> AAQLSEQLAELEKRSGGRLGVAVLDTATGRRIAYRGDERFPMCSTFKALLAAAVLARVDQGKERLDRRITYGKEDLVDYSPVTEKHVGDGMTVAELCEAAITLSDNTAANLLLEALGGPAALTAFLRSIGDEVTRLDRWEPELNEAAPGDPRDTTTPAAMAATLRTLLLGDALSPASRQQLVDWLVANKTGDKRLRAGLPADDRVGDKTGTGGHGTTNDIAVIWPPGRAPIVVTVYLTESQVDADARDAVIAEVGRLVVEAFHHHHHH

Here, we explore and test these notions using resurrected Precambrian β-lactamases11 as scaffolds for the engineering of completely new active sites. Of these systems, resurrected Precambrian β-lactamases have been thoroughly characterized in terms of their structure, function and stability. These putative ancestral proteins have been shown to be highly stable and able to efficiently degrade several antibiotics. A hydrophobic-to-ionizable amino acid replacement generates a buried (or partially buried) residue with the perturbed properties that are useful in catalysis and conformational flexibility assists the generation of a completely new active site by facilitating substrate and transition-state binding. We have shown that, when using resurrected Precambrian β-lactamases as scaffolds for protein engineering, a minimalist design approach based on this mechanism leads to levels of catalysis for the Kemp elimination reaction of up to approximately seven orders of magnitude above the rate of the uncatalysed reaction, as well as to significant ester hydrolysis activity.

Specifically, X-ray crystallography in the presence of 5(6)-nitrobenzotriazole, a known transition-state analogue of the Kemp elimination reaction and inhibition by this analogue support that Kemp elimination does occur at the site generated by the W229D replacement. Following from this, 3D-structure determination in the presence of the transition-state analogue confirms the role of conformational flexibility in the generation of a new function, as transition-state binding is shown to rely on conformational rearrangements. Specifically, the bound transition-state analogue is displaced with respect to the position originally occupied by the tryptophan 229, as required by the presence of an aspartate residue at position 229 in the active variants. Such a displacement is made possible by a shift of the h11 α-helix (and the concomitant shift of the substantially solvent-exposed h1 α-helix). We note also that the catalytic efficiency for the Kemp elimination in the engineered ancestral proteins correlates with the transition-state analogue binding constants derived from inhibition experiments, supporting that catalysis is linked to transition-state stabilization. We subsequently performed MD simulations in the presence of the transition-state analogue 5(6)-nitrobenzotriazole (TSA) to explore the impact of transition-state binding on the conformational dynamics, as well as how well each system could accommodate the transition state in its new active site. The W229D variants of the ancestral scaffolds that give rise to substantial Kemp elimination activity (PNCA, GNCAMP and GNCA4) can accept the TSA in the MD simulations, although the TSA dissociates from the less active W229D variant of the PNCA scaffold after about 50 ns.> SNAMSNNQQMMLNRIKVVLAEKQRTNRWLAEQMG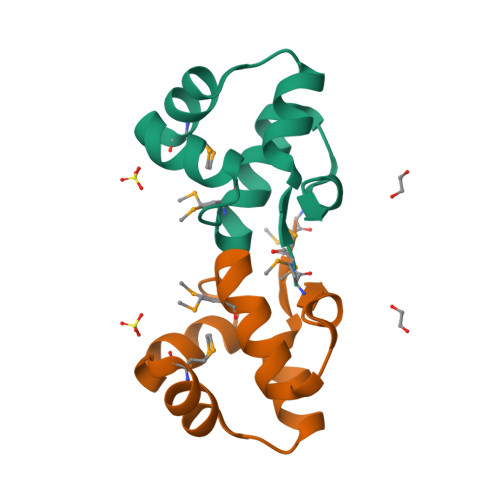KSENTISRWCSNKSQPSLDMLVKVAELLNVDPRQLINGKIKI>MQKRAIYPGTFDPITNGHIDIVTRATQMFDHVILAIAASPSKKPMFTLEERVALAQQATAHLGNVEVVGFSDLMANFAR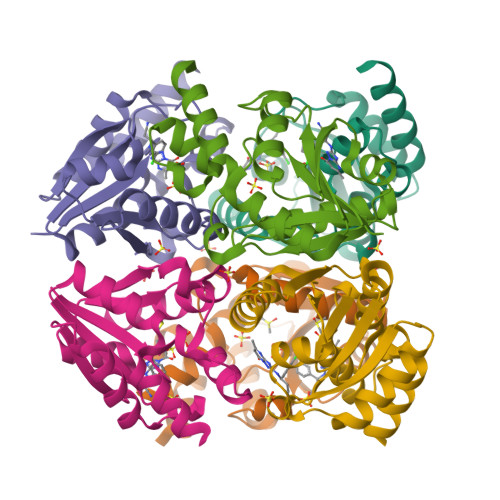NQHATVLIRGLRAVADFEYEMQLAHMNRHLMPELESVFLMPSKEWSFISSSLVKEVARHQGDVTHFLPENVHQALMAKLAVD[2x]>MTDIVYDVEGFRAFLPKETLRWIRHRELERKVGVVEKFSDRVGPIPVEIRRRRSQYGEFYHAGKGTTRIQARVSAAMECVERAAAEPREEIIERGPEGDKWTPAWYRTEPREWVEGVDLTTREPVYVPANEVFHPWLGDALPSHTNGLSAGRLREEAVIQGLLEVVERDSWSIVEYFRIHPPELEVHGELEELRRSLEREVGRVELRLLPSRVEGVYVVGAVTEAERVEEMVMGFGASPDPEMAVLRALLEVAQGLSMARRGIESPVRKGLGEF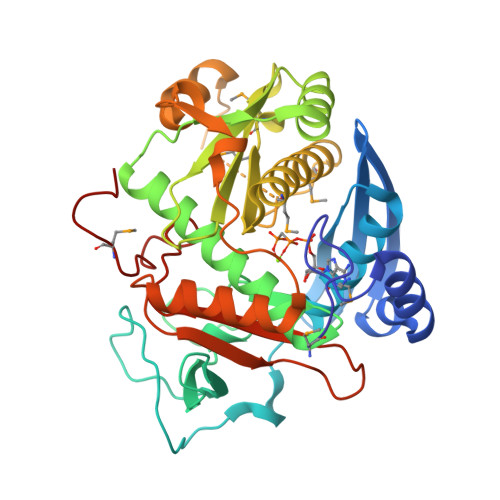SAPGKLTPERLKRLNRHWFEPEGTVEIDDLDRVITTGSLEKLTEELVERVAEAGLGKVIEVDLTLENLDVPVVRVRVTGASEYVIDEARVGNMPEKPPGVPMG[6x]> MIGYL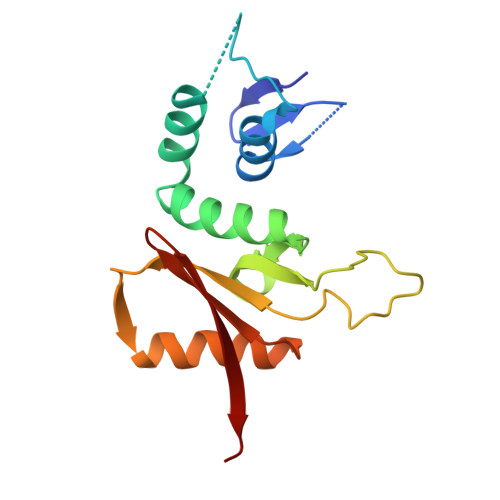FGNRVLVDDKELPLIEAYYLLDKGELEVYEDDKKLSKEEFLKKCLTYDERFLIRYKAYKELRDKGYTLGTALKFGADFRVYDIGVIPKKGKRSEREHSKWVLYPVSKDETFDFYEFASKNRVAHSTRKKMLMGIVSDKIEFIEVSWKKP1-{[(3S,4S)-3-({4-[2-(4-fluorobenzene-1-sulfonyl)ethyl]piperidin-1-yl}methyl)-4-(3-fluorophenyl)pyrrolidin-1-yl]methyl}cyclopentane-1-carboxylic acid | C31 H40 F2 N2 O4 S | 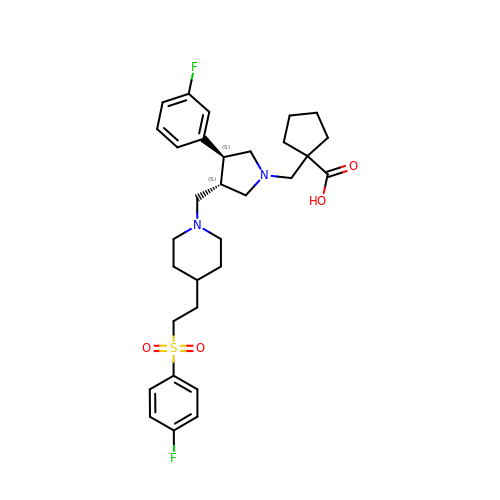JLKKIAYYHXNZIY-ABYGYWHVSA-N>[2x]MRAVNWNKKEDDFSLMFWKQNIAQFWTEEEIAVSSDKNTWVQLSKEEQIAYKRVLGGLTLGDTKQGGEGMPLVLVHLENLQAKSVLAFMGAMEEVHAKSYSHIFTTLATEEEIDEIFDWVDTHPLLEKKAGIITSYYRRLLKPEVTKKELYMAMVASVFLESYLFYSGFFYPLYLAGQGKLTASGEIINLIIRDESIHGVFVGILAQQIFAELSAEDQQEVQKE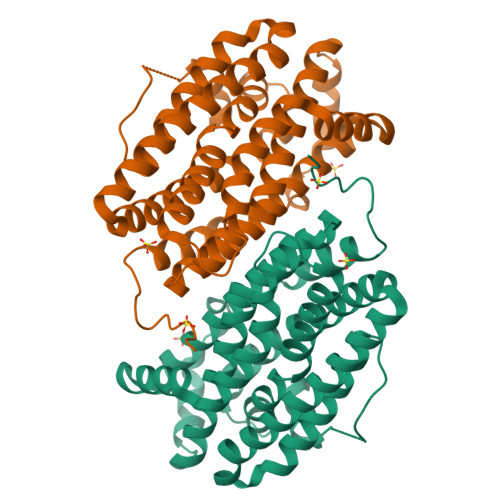TQELLMELYEIEMAYTEEIYTSIGLVEDVNRFVRYNANKGLMNLGLEPKFEEEEINPIVLNGLRTDTKNHDFFSVKGNGYVKATNVEKLSDDDFVFNF2-(5-BENZYLAMINO-2-METHYLSULFANYL-6-OXO-6H-PYRIMIDIN-1-YL)-N-[4-GUANIDINO-1-(THIAZOLE-2-CARBONYL)-BUTYL]-ACETAMIDE | C23 H28 N8 O3 S2 | 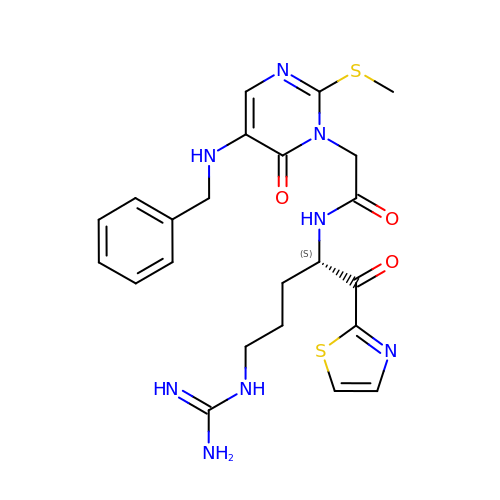NSVPIISNZVMCCY-INIZCTEOSA-N> PIVDTGSVAPLSAAEKTKIR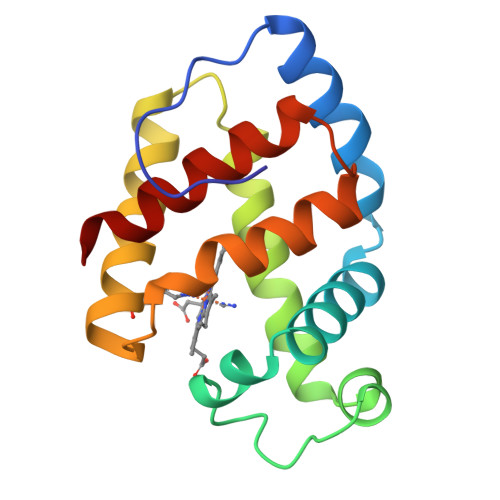SAWAPVYSTYETSGVDILVKFFTSTPAAQEFFPKFKGLTTADELKKSADVRWHAERIINAVDDAVASMDDTEKMSMKLRNLSGKHAKSFQVDPEYFKVLAAVIADTVAAGDAGFEKLMSMICILLRSAY> G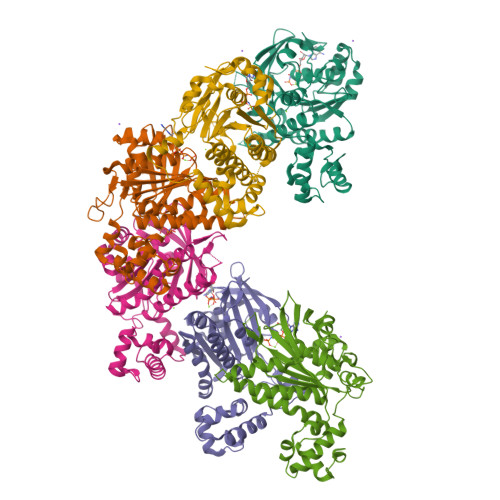LTDLPGVGPSTAEKLVEAGYIDFMKIATATVGELTDIEGISEKAAAKMIMGARDLCDLGFKSGIDLLKQRSTVWKLSTSSSELDSVLGGGLESQSVTEFAGVFGSGKTQIMHQSCVNLQNPEFLFYDEEAVSKGEVAQPKAVYIDTEGTFRPERIMQMAEHAGIDGQTVLDNTFVARAYNSDMQMLFAEKIEDLIQEGNNIKLVVIDSLTSTFRNEYTGRGKLAERQQKLGRHMATLNKLADLFNCVVLVTNQVSAKPDAFFGMAEQAIGGHIVGHAATFRFFVRKGKGDKRVAKLYKSPHLPDAEAIFRITEKGIQD>[2x]GSMTDGDYDYLIKLLALGDSGVGKTTFLYRYTDNKFNPKFITTVGIDFREKRVVYDTQGADGASGKAFKVHLQLWDTAGLERFR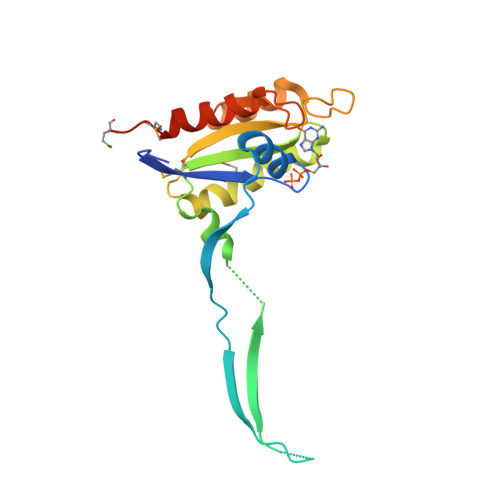SLTTAFFRDAMGFLLMFDLTSQQSFLNVRNWMSQLQANAYCENPDIVLIGNKADLPDQREVNERQARELAEKYGIPYFETSAATGQNVEKSVETLLDLIMKRMEKCVEKTQ>MAATRTRGYVTTKDGIKWYYEQEGSGPDVVLIPDGLGECQMFDKPMSLIASNGFRVTTFDMPGMSRSSDAPPETYQDITGRKLAGYIITLLDTLDIKIASVWGCASGAST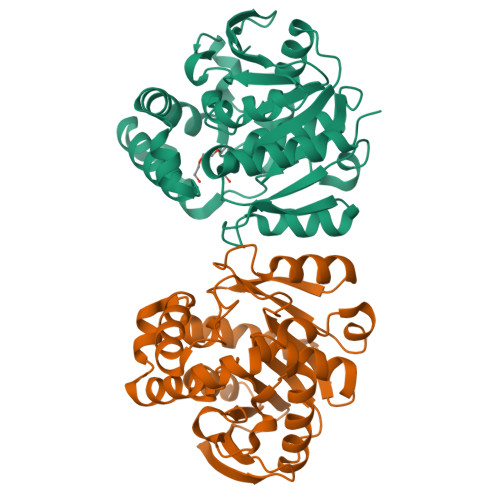VLALCSDYPERVRNGMPHEVPTENPDILLHIHEVDPATISQEMAANSRAYSGNVEAWDALGPEVHARLHDNYPRWAYGYPRTIPPSAPVKTEDLHKVPIDWTVGASTPTKLFFENIVIAAREGINIGTLPGNHFPYVSHPEEFAKYVVETSRKYLK[8x]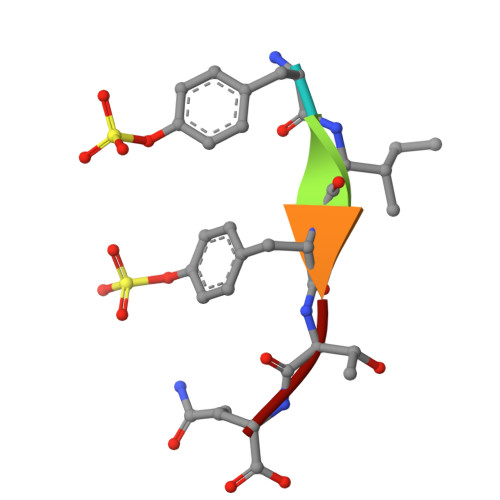> YIYTQ>ANLERTFIAIKPDGVQRGLVGEIIKRFEQKGFRLVAMKFLRASEEHLKQHYIDLKDRPFFPGLVKYMNSGPVVAMVWEGLNVVKTGAVMLGETNPADSKPGTIRGDFCIQVGRNIIHGSDSVKSAEKEISLWFKPEE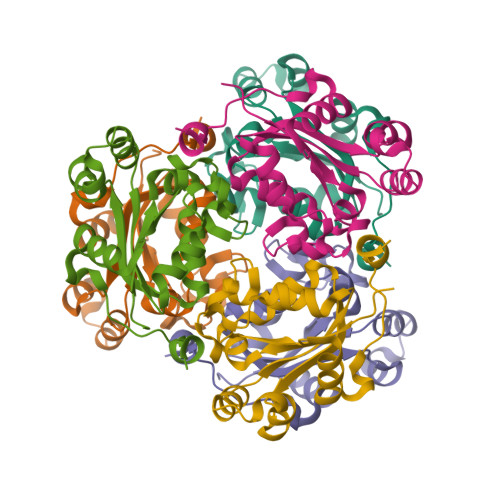LVDYKSCAHDWVYE[6x]> MVLFTRCEKARKEKLAAGYKPLVDYLIDCDTPTFLERIEAIQEWDRSRDDLYVWIPILDRMDGLLLKVAEKYKYKQDPKKECEVKLVEMEAHDVDYCLKMLKFTRRLLLNTENRFVYSSGDVLMYLLNCPNFTIKLAVMRILAILGERFVIAREKIVAHNIFGDHNLRKKTLKLALSLSSSVMDEDGEHFSLVDLYFDKKKVPQKWRKLRFTHYTSNDFKKSSQQKNNINETQTSIKKVTMTTQELCEHSLQQIFDKGMALLPAESWFDFSIKASVAKAFSDDSGENIDLRNIIIETKLNAIAFVNTIFSPPQVSSKLFELDPYAFNSLTDLISLSETKIPKELRTDALFTLECISLKHVWCSDIIRNLGGNISHGLLFQILRYIAKTLREATDEIDEEYNVRFFYLISNLADVKPLHESLFAAGLIPTLLEIVSIRNCPYKRTLASATHLLETFIDNSETTTEFIENDGFTMLITSVANEIDFTLAHPETWQPPKYSVVYYSISFRELAYIRSLLKLVLKLLSTDSGDRIRNLIDSPILVSLKKILENKLVFGLTLITYTLDVVQKVINSEPTIYPVLVEAGLIPYVIDNFPKLIGPSAELLSLLPDVVSAICLNPEGLKQVKEKGLINNLFDFLLDADHARILTGGDRSTEYGTDIDELARHYPDLKANIVEALCNVIRKMPSTFRNEREFLFTSPKDQKYFFHRKNEEILTDKEEHEPAYWELLDKGTMLDTFTSVLFGMSLGNGSFSQVPQHLEARDFLAIIFMENPPYEYFTSVAISNVTEVLQYLDEKYEDYAFMDVMKVLNDQLENLNDFLNSPNDRSFFLERDGENSVRSCHSKLCRLAAILNIVTNVYIDLTTLSCKRIMQIYSYFDKRGFSLIKNLKLLFQKCALEEMYIRQHMPDSVITETMPLPIVDVSGDGPPLQIYIDDPKKGDQKGKITSVKTRNTLQMRTILYTLQSNTAILFRCFLRLSHSRNMDLEHKDLTTEVHIFENVVENVIEMLKATELEGHLPYILVLLNFNTFVFTIPKASPNSTEILQTIPAYIFYQKGGYLLYLHIIRDLFTRMTKIKDLSSLDNINYIDESNGILTLSCLINALTFYNKSMQTETMENVQSIGKYYVSIDDDYNIMKALTVPIKVMALAMILDLDKSDSLFKTQSRNVPYSVFKQLLSMLKNIFTNVNIYTKELYELHWDLIFPPIKKISLFEQVGIPGDVAANYLTDTGDDLPADNSIGLFSPEQWEKYKKLIGEDKSIYYPQPMQAQYYKGCSSKELDELRDTFFNDGLPSRIFTVLPFYPKLVNAFAKTLLQIFTKYDEPTEVFAGRILDRILETDLDDPATLSSLIHLFGIFLNEKYIYQKASHLMQRFIEYLEKSLKPEHVNTPWFSKALYVYEIILAKSELPHLEELSKDVLLRYPLLSMAKVFRIPDPMKQKLFDILIRVSDISNFYSALATSRILIFYSRDELYANNIARSGILSRLLKVIGSFQKLDKINFLESSFLLLTRRCFETTENVDALIRAEINRSFTARPLGGGDDAVRELTTILEEKAHVVMRSPSQFIDVLCETARFHEFDDQGALVDYSLKRFLGEKDKNTQASSTEKSDIYERTGIMHLLLSQLMAASEKDWLSEPANSSDLPENKKAQLDPSRNPVCAYMIFLLKLLVELVSSYNQCKFEFLTFSRRNTYAERPRPRTTAINFFLYRLLDKPVGTDHDKHEAKRREVIGMLARSVIIGFLATVQDDRTTKTDVKLADPHMNFIRKFAIEAIIKAIRNATSSSKLLESNHLKLDMWFRIITSMVYVQAPYLRQLLDSNKVEADQYQLCKLVIDLGLPSVITEAMASIDLNYPFSKKIFNVAVEALNTISSTRNNFSEHFKIEDHDEVEDEVDESDKEEIPDMFKNSALGMYDVEDIEEDDDDDTSLIGDDDAMAFVDSDNGFEVVFSDEDDDMGEEDADDARSDSEENELSSEMQSSTADGTDVDYEVDDADGLIINIDQPSGDDEEMADYDANISHSSHSENEDDASMDVIEVYDDELSSGYDVDLSDYDVDESDWDSGLSSLSISDEDSESSEDEPINSTRMGDSRRRWLIAEGVELTDDSQGESEEDDRGVFRGIEHIFSNENEPLFRVHDEMRHRNHHRSINRTHFHSAMSAPSLSLLNRGRRNQSNLINPLGPTGLEQVENDISDQVTVAGSGSRPRSHHLHFSEVLVSGSFFDEPVLDGIILKSTVSRWKDIFDMFYDSKTYANCIIPTVINRLYKVSLALQKDLENKREQEKLKNKNLLFNEAKVESHNSSDAISVEQDDIQESNVTHDDHEPVYVTIQGSEVDIGGTDIDPEFMNALPDDIRADVFAQHVRERRAEARLNSDHNVHSREIDSDFLEAIPEDIREGILDTEAEEQRMFGRIGSSADVIRADDDVSNNDEEVENGLDHGNSNDRNNADPEKKKPARIYFAPLIDRAGIASLMKSVFISKPYIQREIYHELFYRLCSSKQNRNDLMNTFLFILSEGIIDQHSLEKVYNIISSRAMGHAKTTTVRQLPSDCTPLTVANQTIEILQSLIDADSRLKYFLIAEHDNLIVNKANNKSRKEALPDKKLRWPLWHLFSLLDRKLITDESVLMDLLTRILQVCTKTLAVLSTSSNGKENLSKKFHLPSFDEDDLMKILSIIMLDSCTTRVFQQTLNIIYNLSKLQGCMSIFTKHLVSLAISIMSKLKSALDGLSREVGTITTGMEINSELLQKFTLPSSDQAKLLKILTTVDFLYTHKRKEEERNVKDLQSLYDKMNGGPVWSSLSECLSQFEKSQAINTSATILLPLIESLMVVCRRSDLSQNRNTAVKYEDAKLLDFSKTRVENLFFPFTDAHKKLLNQMIRSNPKLMSGPFALLVKNPKVLDFDNKRYFFNAKLKSDNQERPKLPITVRREQVFLDSYRALFFKTNDEIKNSKLEITFKGESGVDAGGVTREWYQVLSRQMFNPDYALFLPVPSDKTTFHPNRTSGINPEHLSFFKFIGMIIGKAIRDQCFLDCHFSREVYKNILGRPVSLKDMESLDPDYYKSLVWILENDITDIIEETFSVETDDYGEHKVINLIEGGKDIIVTEANKQDYVKKVVEYKLQTSVKEQMDNFLVGFYALISKDLITIFDEQELELLISGLPDIDVDDWKNNTTYVNYTATCKEVSYFWRAVRSFDAEERAKLLQFVTGTSKVPLNGFKELSGVNGVCKFSIHRDFGSSERLPSSHTCFNQLNLPPYESYETLRGSLLLAINEGHEGFGLALEVLFQGP

Tom1p is a large, 374 kDa member of a broadly conserved family of HUWE1 factors (also called Mule, Lasu, Ureb1, Arf-BP1, HectH9/E3^Histone^, Ptr1, Upl1, or Eel-1;). This family is characterized by a large N-terminal domain attached to a smaller C-terminal HECT domain (Homologous to E6-AP Carboxyl Terminus) that provides ubiquitin ligase activity ([Fig fig1]). Tom1p has been implicated in the turnover of excess levels of small, basic proteins including ribosomal components and histones. We determined cryo-EM structures of Tom1p to reveal a helical repeat solenoid architecture for the 2,888 residues preceding the C-terminal HECT domain and an overall architecture that resembles the published structures of HUWE1 but with a larger fraction of ordered residues.

We performed single-particle cryo-EM reconstructions of two Tom1p constructs: full-length Tom1p that contained a 20-residue tag including 12 histidines inserted between residues K1074-D1075 (Tom1p^His^; physiologically active in all phenotype assays) and Tom1p^ΔAD^ with the C-terminal Protein A described for intact Tom1p above ([Fig fig2], presumably inactive). These structures were determined at resolutions of 3.97 Å (Tom1p^His^) and 3.07 Å (Tom1p^ΔAD^) for the dominant closed ring conformations ([Fig fig6], 7C, S6). The two maps and structural models were very similar to each other, indicating that neither the internal affinity tag, the absence of the acidic domain, or the presence of a C-terminal Protein A scar induced notable conformational changes. Unless otherwise noted, the higher resolution Tom1p^ΔAD^ map was used for descriptions and illustrations herein. 2,792 (85%) of the 3,268 Tom1p residues were modeled into Tom1p^ΔAD^, which corresponds to 96% of the residues in Tom1p^ΔAD^ ([Fig fig6]). Beginning and end points of missing density in Tom1p^ΔAD^ structure: 214-235, 1873-2219 (region containing acidic domain), 2276-2316, 2399-2449, 2575-2589. The Tom1p acidic domain (residues 1873-2131), which is conserved in HUWE1, is found within a larger disordered region (residues 1871-2219), the ends of which are located on the inner face of the solenoid, suggesting that this unstructured component of Tom1p will at least partially occupy the basket ([Fig fig6], 6C). We therefore deleted the 259-residue acidic domain (Tom1p^ΔAD^; lacking E1873-E2131; 38% D, E, 4% K, R, pI 3.0) and found that the resulting protein no longer bound Spt6p^tSH2^ in the far-western assay ([Fig fig2]). Tom1p^ΔAD^ was expressed at the normal level in yeast and the purified protein was well-behaved ([Fig fig2]), so deletion of the acidic domain did not destabilize Tom1p but did substantially reduce the affinity for Spt6p^tSH2^. Binding was not observed with Tom1p^ΔAD^ but complexes formed normally when just the Spt6p^tSH2^ binding site was removed in Tom1p^Δ11^ ([Fig fig4]).> MTRLTVALSGACMVTRGGLITSDPAAERLRDLLRGTDFAVTNLEVVPSDGRGHPVHNAVGGGCLIADSAVLDEVTAAGFSVLGCANNHAMDLGTEGVLGTMDLLRARGIPYAGIGADLTGARRPVYADRPGGSLALLSCTATFLPGQEAADPSPELPGRPGLNPLRHTATMQVTADQMDVLRTIDAETGLRARRAEARALLGVDPALLGPDRLALFGTRFRTADAPGFTTECDPRDLDEIARWVGEARLRADLVVVSVHSHEPGPTPETPGEFLRVFAHRMIDEGAHAVVGHGPHFLRGVELYRNKPIFYSLGNIVSQIELTDRVSAEDYAKVTAERPLTPGRYYDRLSGHGTRLFAPHRRYWQSLVPVLTFEDGTLTAARLHPVDLGFGRPVHRRGRPRLADRAEAEKTLTDVAQLSQPYGTAIEVMDDGTGELALDVA

The lasso peptide MS-271 is a ribosomally synthesized and post-translationally modified peptide (RiPP) consisting of 21 amino acids with D-tryptophan at the C-terminus, and is derived from the precursor peptide MslA. MslH, encoded in the MS-271 biosynthetic gene cluster (msl), catalyzes the epimerization at the Cα center of the MslA C-terminal Trp21, leading to epi-MslA. Herein, based on X-ray crystallographic studies in association with MslA core peptide analogues, we show that MslH is a metallo-dependent peptide epimerase with a calcineurin-like fold. The crystal structure analysis, followed by site-directed mutagenesis, docking simulation, and ICP-MS studies demonstrate that MslH employs acid/base chemistry to facilitate the reversible epimerization of the C-terminal Trp21 of MslA, by utilizing two pairs of His/Asp catalytic residues that are electrostatically tethered to a six-coordination motif with a Ca(II) ion via water molecules.

The in vitro experiment revealed that all variants lacked epimerase activity, indicating that the four residues are crucial for catalysis. In contrast, the loss of catalytic activity of the His295N and Asp11A variants could be due to a structural collapse of the metal-binding and substrate-binding sites, caused by a breakdown of the hydrogen bonding network between six-coordination motif and Asp11/His295 via the w2 water molecule and substrate. Therefore, we evaluated the His295N and Asp11A variants from a structural aspect. We obtained their crystal structures, MslH Asp11A:apo and MslH His295N:apo at 2.41 and 2.55 Å resolutions, respectively. Both crystal structures indicated that the variants retained the same six-coordination motif as that in the wild-type MslH crystal structure. The His295N substitution had no effect on the active center organization, while the Asp11A substitution led to the flexibility of His295 in the MslH Asp11A:apo crystal structure, where a 1:1 alternative state was observed for the His295 residue. The main chain carbonyl group of the Pro294 residue in the MslH Asp11A:apo crystal structure was inverted by 180 degrees, as compared with that of the wild type. Moreover, the comparison of the MslH His295N:apo structure with the MslH:MslA Trp21G complex structure showed that the distance between the Cα center of MslA Gly21 and Oδ of Asn295 atom is 4.5 Å, which is longer than that (3.4 Å) in the MslH:MslA Trp21G structure. These observations suggested that the Asp11 and His295 residues would play important roles in maintaining the appropriate catalytic state of MslH.> XRMKQIEDK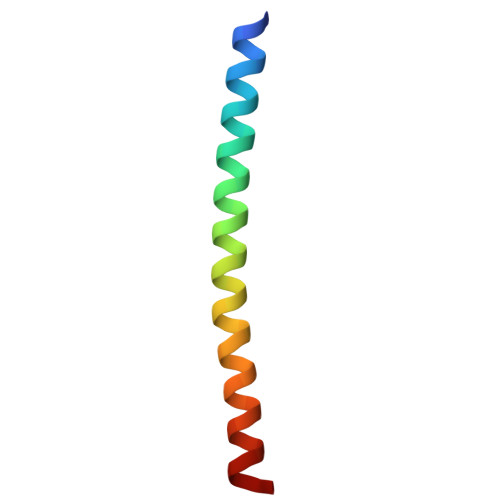IEEIESKQKKIENEIARIKKLLQLTVWGIKQLQARIL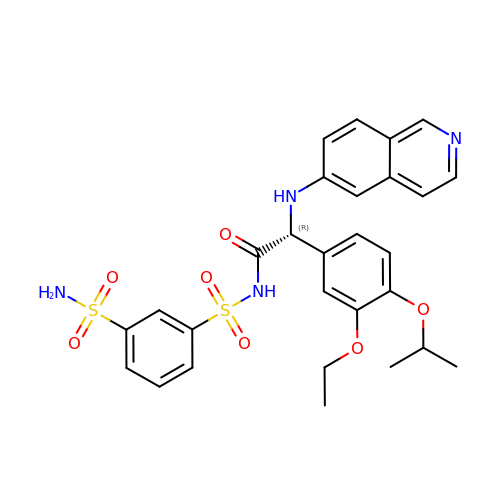(2R)-2-[3-ethoxy-4-(propan-2-yloxy)phenyl]-2-(isoquinolin-6-ylamino)-N-[(3-sulfamoylphenyl)sulfonyl]ethanamide | C28 H30 N4 O7 S2 | QHVDUHFNSHQJRC-HHHXNRCGSA-N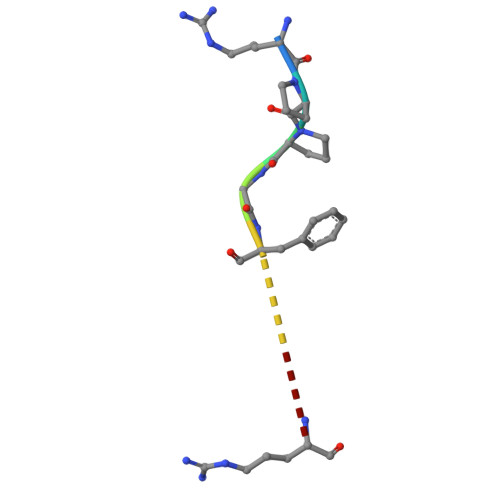> RPPGFSPFR> SNAMFAPQGLAQFIKVNVTLENGEPVFIYTDANGQVCQGDITVTQAGTITYLLNDQTLKGLKFVGVGFVTPFDGIIDAVTISSDGMLVQLVDLDKTPGTTKFQFVLSNTANTL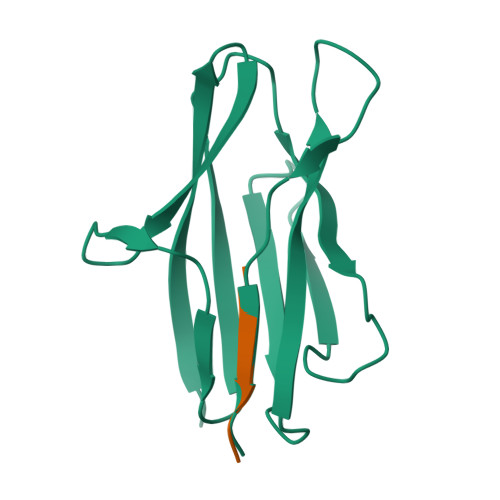LVLAPDPQIINRPQN;> PQIINRPQN> AGFGAQHRKMGKSLYLRNEVFAAWIEKVDALVQDELGYSVLELILDDAQDYGIETTQVTIFAIQIALGELLRHHGAKPAAVIGQSLGEAASAYFAGGLSLRDATRAICSRS

Recently, powerful evidence has verified that Pks13 is an essential enzyme in the mycolic acid biosynthesis pathway, and Pks13 has been extensively studied as a drug target for TB. The type-1 polyketide synthase enzyme Pks13 consists of five domains. The overall Pks13 topological structure has the order ACP-KS-AT-ACP-TE. The meromycoloyl chain on the N-ACP domain is transferred to the KS domain, and the intermediate product α-alkyl β-ketothioester is produced by a Claisen-type condensation reaction with another substrate, the carboxyacyl-CoA loaded by the AT domain.

We have determined the 2.59 Å high-resolution crystal structure of a partial AT domain from the M. tuberculosis Pks13 protein. Then, the crystals were solved, and the N-terminal sequence was identified by mass spectrometry, the results of which were in line with the phase presented by the Se-Met crystal dataset. These results indicated that the crystallized protein was actually proteolyzed to become a fragment (Ala717 to Arg826). The overall structure of the core motif contains a long α helix, five short α helixes and two short η turns, in the order of α1-α2-α3-α4-η1-η2-α5-α6, which constitutes a compact motif. The crystallized core motif ranging from Leu717 to Arg826 represents approximately one-third of the AT domain, and the overall crystal structure displays a fold similar to the reported AT domain. Although sequence alignment showed 100% identity between the core motif and the AT domain, the secondary structure elements presented a slight conformational change from residues Ala796 to Ser801, for which refinement indicated two η turns instead of the β strand highlighted by red dashed square line. In our work, the topographic conformation of Ala796 to Ser801 was transformed into two relatively disordered η turns, along with the conformational change of the position of Ser801 dislocating from the substrate. Furthermore, the side chain of the binding site Arg826 was also stretched to the reverse side of α5 and lost its interaction with Gln773. According to a close view of the superimposition, some particular apolar contacts among α1 (His723, Leu730) and the long α4 (Gln773, Ile779, Gln780, and Leu783) and α5 (Ile823) residues all contribute to the stabilization of the unique state. The nucleophilic elbow of α10 and β5 also transformed from an electropositive state to an electronegative state which indicates an unsuitable state to absorb a substrate. In summary, the conformational change of residues from Ala796 to Ser801 and the rearrangement of residues Gln773, Ser801, and Arg826 might all suggest that the degraded fragment formed a unique crystal packing state to survive proteolysis.> MNNNDLVAKLWKLCDNLRDGGVSYQNYVNELASLLFLKMCKETGQEAEYLPEGYRWDDLKSRIGQEQLQFYRKMLVHLGEDDKKLVQAVFHNVSTTITEPKQITALVSNMDSLDWYNGAHGKSRDDFGDMYEGLLQKNANETKSGAGQYFTPRPLIKTIIHLLKPQPREVVQDPAAGTAGFLIEADRYVKSQTNDLDDLDGDTQDFQIHRAFIGLELVPGTRRLALMNCLLHDIEGNLDHGGAIRLGNTLGSDGE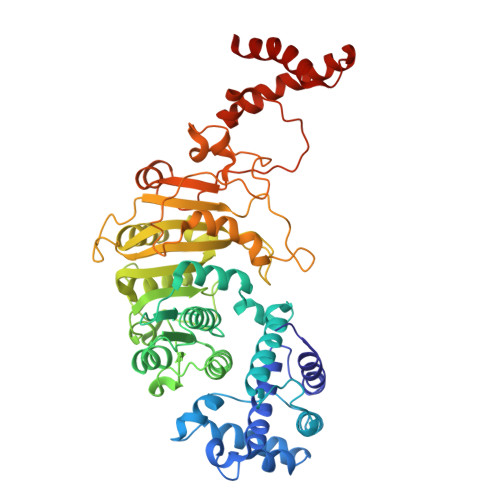NLPKAHIVATNPPFGSAAGTNITRTFVHPTSNKQLCFMQHIIETLHPGGRAAVVVPDNVLFEGGKGTDIRRDLMDKCHLHTILRLPTGIFYAQGVKTNVLFFTKGTVANPNQDKNCTDDVWVYDLRTNMPSFGKRTPFTDEHLQPFERVYGEDPHGLSPRTEGEWSFNAEETEVADSEENKNTDQHLATSRWRKFSREWIRTAKSDSLDISWLKDKDSIDADSLPEPDVLAAEAMGELVQALSELDALMRELGASDEADLQRQLLEEAFGGVKE>[2x]MQDNSRYTHFLTQHYDAKPQGRDDRYCESIMRRRGLTSPCKDINTFIHGNKRSIKAICENKNGNPHRENLRISKSSFQVTTCKLTTPSPQNISNCQYRATAGFRNVVVACENGLPV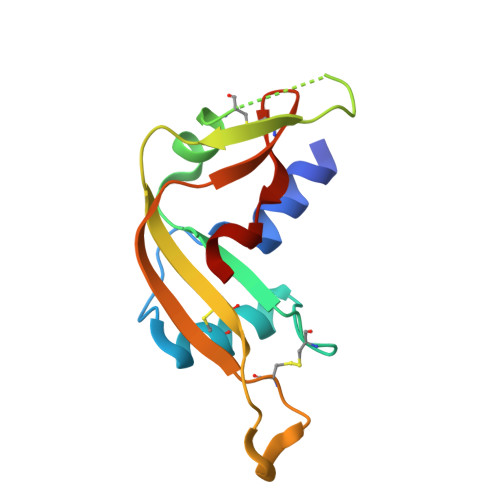HLDQSIFRRP>MDTEKLMKAGEIAKKVREKAIKLARPGMLLLELAESIEKMIMELGGKPAFPVNLSINEIAAHYTPYKGDTTVLKEGDYLKIDVGVHIDGFIADTAVTVRVGMEEDELMEAAKEALNAAISVARAGV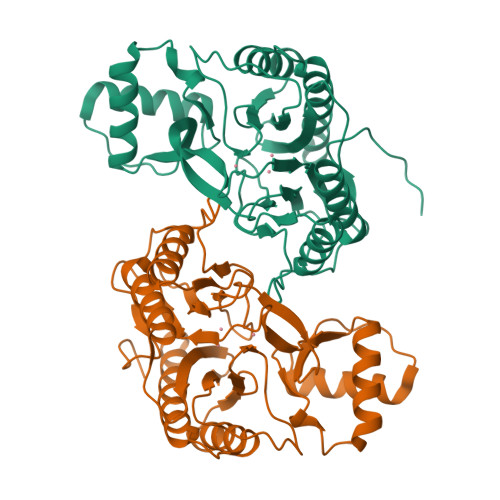EIKELGKAIENEIRKRGFKPIVNLSGHKIERYKLHAGISIPNIYRPHDNYVLKEGDVFAIEPFATIGAGQVIEVPPTLIYMYVRDVPVRVAQARFLLAKIKREYGTLPFAYRWLQNDMPEGQLKLALKTLEKAGAIYGYPVLKEIRNGIVAQFEHTIIVEKDSVIVTQDMINKST[2x]>[2x]TGGVQTVTLIPGDGIGPEISAAVMKIFDAAKAPIQWEERNVTAIQGPGGKWMIPSEAKESMDKNKMGLKGPLKTPIAAGHPSMNLLLRKTFDLYANVRPCVSIEGYKTPYTDVNIVTIRENTEGEYSGIEHVIVDGVVASIKLITEGASKRIAEFAFEYARNNHRSNVTAVHKANIMRMSDGLFLQKCREVAESCKDIKFNEMYLDTVCLNMVQDPSQFDVLVMPNLYGDILSDLCAGLIGGLGVTPSGNIGANGVAIFESVHGTAPDIAGKDMANPTALLLSAVMMLRHMGLFDHAARIEAACFATIKDGKSLTKDLGGNAKC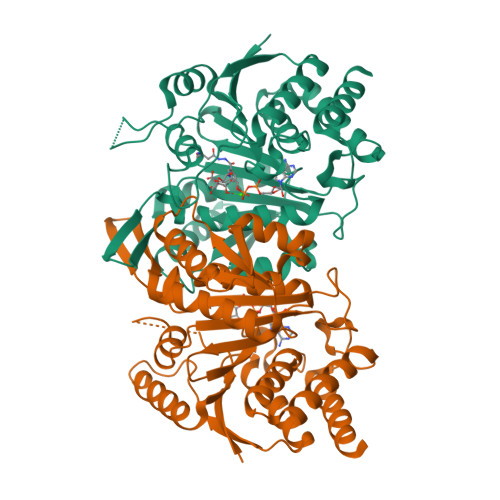SDFTEEICRRVKDLD;>[2x]ASRSQAEDVRVEGSFPVTMLPGDGVGPELMHAVKEVFKAAAVPVEFQEHHLSEVQNMASEEKLEQVLSSMKENKVAIIGKIHTPMEYKGELASYDMRLRRKLDLFANVVHVKSLPGYMTRHNNLDLVIIREQTEGEYSSLEHESARGVIECLKIVTRAKSQRIAKFAFDYATKKGRGKVTAVHKANIMKLGDGLFLQCCEEVAELYPKIKFETMIIDNCCMQLVQNPYQFDVLVMPNLYGNIIDNLAAGLVGGAGVVPGESYSAEYAVFETGARHPFAQAVGRNIANPTAMLLSASNMLRHLNLEYHSSMIADAVKKVIKVGKVRTSDMGGYATCHDFTEEICRRVKDLDEN> MAKLGIHSNDTRDAWVNKIAQLNT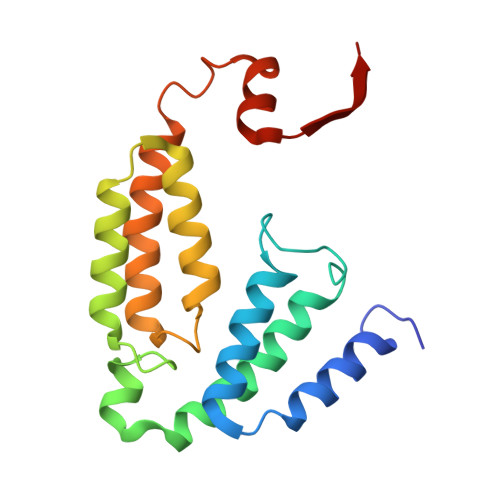LEKAAEMLKQFRMDHTTPFRNSYELDNDYLWIEAKLEEKVAVLKARAFNEVDFRHKTAFGEDAKSVLDGTVAKMNAAKDKWEAEKIHIGFRQAYKPPIMPVNYFLDGERQLGTRLMELRNLNYYDTPLEELRKQRGVRVVHLQSPH>[2x]HGSMISEIIKDRAKLVNEKIEELLKEQEPEGLYRAARHYLKAGGKRLRPVITLLSAEALGEDYRKAIHAAIAIETVHNFTLVHDDIMDEDEMRRGVKTVHTLFGIPTAILAGDTLYAEAFEILSMSDAPPENIVRAVSKLARVCVEICEGQFMDMSFEERDSVGESEYLEMVRKKTGVLIGISASIPAVLFGKDESVEKALWNYGIYSGIGFQIHDDL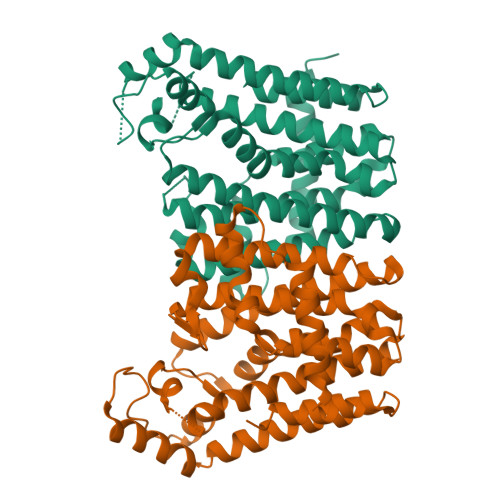LDISGKGKIGKDWGSDILEGKKTLIVIKAFEEGIELETFGKGRASEEELERDIKKLFDCGAVDYARERAREYIEMAKKNLEVIDESPSRNYLVELADYLIERDH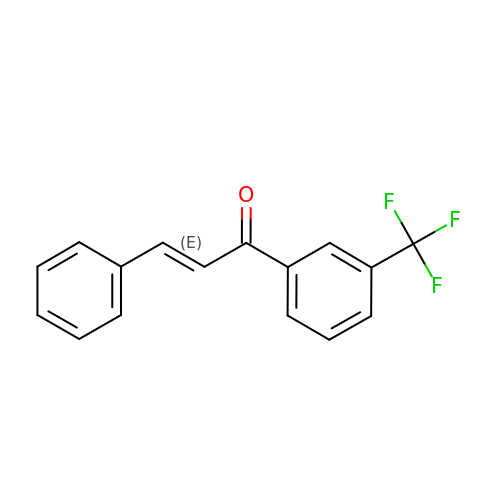(E)-3-phenyl-1-(3-(trifluoromethyl)phenyl)prop-2-en-1-one | C16 H11 F3 O | PBGSCTPDAVCTBJ-MDZDMXLPSA-N> MHHHHHHMKEIAVTIDDKNVIASVSESFHGVAFDASLFSPKGLWSFVDITSPKLFKLLEGLSPGYFR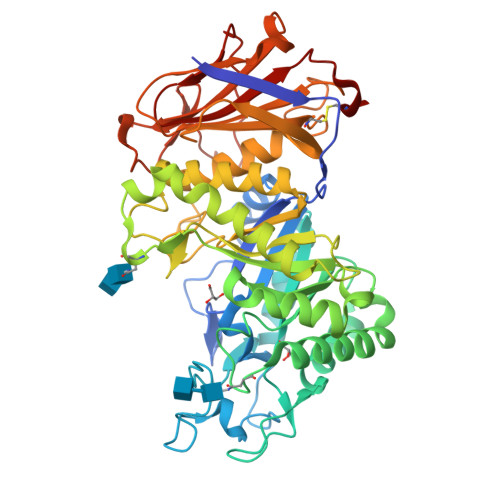VGGTFANWLFFDLDENNKWKDYWAFKDKTPETATITRRWLFRKQNNLKKETFDDLVKLTKGSKMRLLFDLNAEVRTGYEIGKKMTSTWDSSEAEKLFKYCVSKGYGDNIDWELGNEPDHTSAHNLTEKQVGEDFKALHKVLEKYPTLNKGSLVGPDVGWMGVSYVKGLADGAGDHVTAFTLHQYYFDGNTSDVSTYLDATYFKKLQQLFDKVKDVLKNSPHKDKPLWLGETSSGYNSGTKDVSDRYVSGFLTLDKLGLSAANNVKVVIRQTIYNGYYGLLDKNTLEPNPDYWLMHVHNSLVGNTVFKVDVSDPTNKARVYAQCTKTNSKHTQSRYYKGSLTIFALNVGDEDVTLKIDQYSGKKIYSYILTPEGGQLTSQKVLLNGKELKLVSDQLPELNADESKTSFTLSPKTFGFFVVSDANVEACKK> MEPFGTDERNWTHEEKDIITRFLKYDKHVNLKTAEMVYSAEVESAYFGKAGALAGGVISALFFNFPIVRNLPIIRRSVIGVLPFLYCYTWGKNTQEELRWLKTFAAY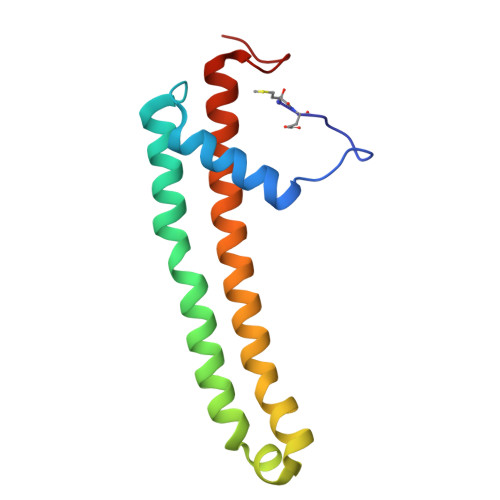QRFVVYHGQHCKLWV>ENLYFQGHMSTLSTHILDISTGTPAEGVTVSLSREGETLANLVTNAQGRIATFSAAPLPAGRYCLTAETGAWFARAGRESVFTRAQIDFVIGEAAEDH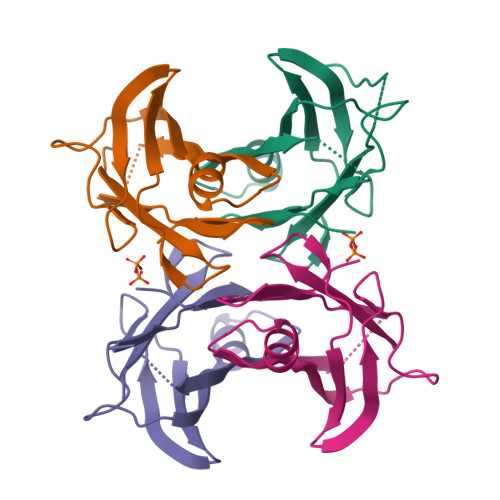FHLPFLIAPGGWSTYRGS[4x]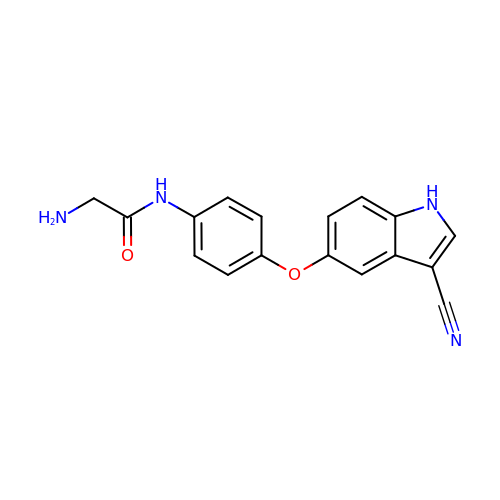2-azanyl-N-[4-[(3-cyano-1H-indol-5-yl)oxy]phenyl]ethanamide | C17 H14 N4 O2 | FTYQKBVNGALNLT-UHFFFAOYSA-N1-[4-chloranyl-3-(trifluoromethyl)phenyl]-3-[[(2R,3S)-5-[5-methyl-2,4-bis(oxidanylidene)pyrimidin-1-yl]-3-oxidanyl-oxolan-2-yl]methyl]thiourea 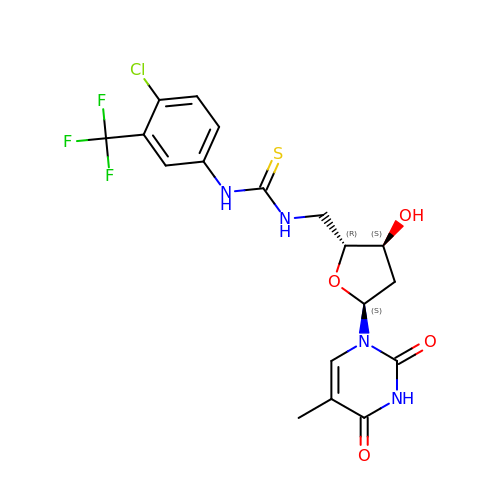| C18 H18 Cl F3 N4 O4 S | IJDGQXGQAWBJEG-MJBXVCDLSA-N>MDYRQLHRWDLPPEEAIKVQNELRKKIKLTPYEGEPEYVAGVDLSFPGKEEGLAVIVVLEYPSFKILEVVSERGEITFPYIPGLLAFREGPLFLKAWEKLRTKPDVVVFDGQGLAHPRKLGIASHMGLFIEIPTIGVAKSRLYGTFKMPEDKRCSWSYLYDGEEIIGCVIRTKEGSAPIFVSPGHLMDVESSKRLIKAFTLPG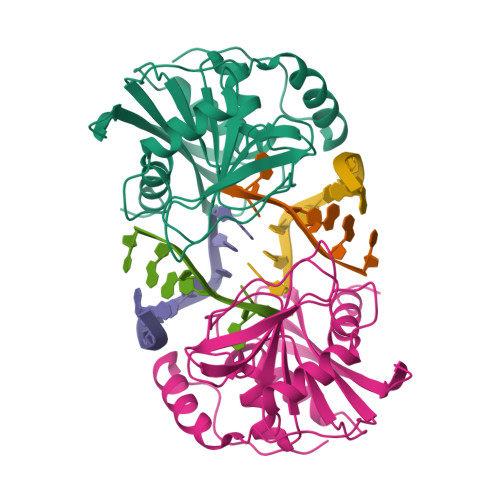RRIPEPTRLAHIYTQRLKKGLF[2x]> GMGLGYGSWEIDPKDLTFLKELGTGQFGVVKYGKWRGQYDVAIKMIKEGSMSEDEFIEEAKVMMNLSHEKLVQLYGVCTKQRPIFIITEYMANGCLLNYLREMRHRFQTQQLLEMCKDVCEAMEYLESKQFLHRDLAARNCLVNDQGVVKVSDFGLSRYVLDDEYTSSVGSKFPVRWSPPEVLMYSKFSSKSDIWAFGVLMWEIYSLGKMPYERFTNSETAEHIAQGLRLYRPHLASEKVYTIM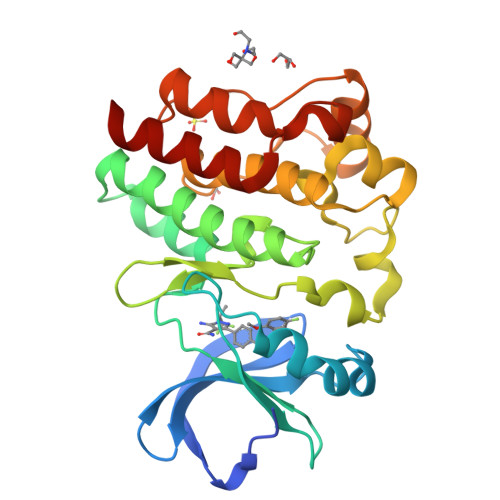YSCWHEKADERPTFKILLSNILDVMDEES> GSHM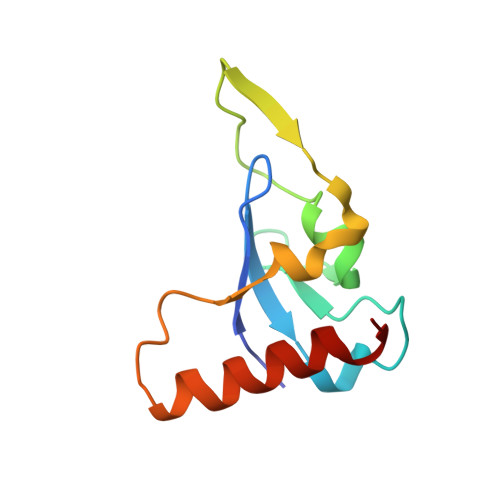RVYHECFGKCKGLLVPELYSSPSAACIQCLDCRLMYPPHKFVVHSHKALENRTCHWGFDSANWRAYILLSQDYTGKEEQARLGRCLDDVKEKFDY>[4x]MSDSLLVRTSRDGDQFHYLWAARRALRLLEPQSTLVALTIEGASTTEMGSQPVVEDGEELIDIAEYYGSNELATATTVRYMQLKHSTMHSDTPFPPSGLQKTIEGFATRYKALIQKIPVETLRTKLEFWFVTNRPVSSSFSEAINDAANQHVTRHPHDLAKLEKFTGLQGAELSIFCQLLHIEGQQDDLWSQRNILLRESAGYLPDLDTEAPLKLKELVNRKALTESAANPSITRMDVLRALGVDETDLFPAPCRIERIENSVSRTQEATLVQRVVEAFGAPVIIHADAGVGKSIFSTHIEEHLPTGSVSILYDCFGLGQYRNASSYRHHHRTALVQMANEMASRGLCHPLIPNAGTG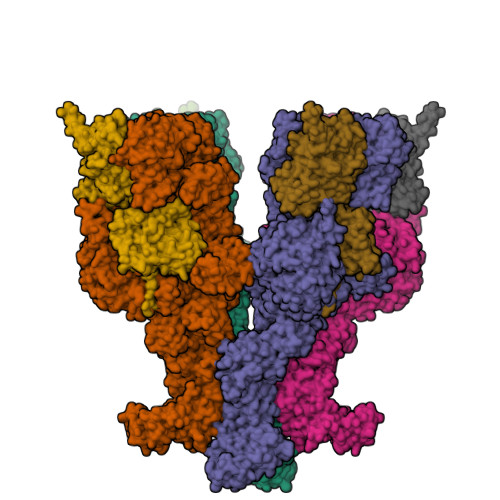ISQYMRAFLHRLSQSISILRASEPLAVLCIIIDAADNAQMAAEEIGETRSFIKDLIREKLPDGVCLVALCRPYRRELLDPPPEALTLSLQTFNRDETAAHLHQKFPDASESDVDEFHRLSSCNPRVQALSLSQNLPLNDTLRLLGPNPKTVEDTIGEVLEKSIARLRDTAGISERAQIDTICSALAILRPLIPLSVLSAISGVAGSAIKSFALDLGRPLIVSGETIQFFDEPAETWFQRRFRPSAADLHQFITKLRPLTKDSSYAASVLPALMLEGNQLSELIELAISSQALPETSAVERRDIELQRLQFALKAALRTGRYQDAAKLALKAGGECAGDNRQRVLLRDNIDLAAKFVGSNGVQELVSRNAFPDTGWPGSRNAYYAAILSEYPELSGEARSRLRLTMEWLTNWSQLPDDERSRQNVTDQDRAVMLIACLNIHGAEAAARELRRWRPRKLSFDAGKIVAMQLLAHARYDELDQLAIAAGNDISLVMGIVLEARKLHRPVAEQAIRRTWRLLKSQRVSIKDRNHANNQTIAAITGMVEMALIQSVCTESESIQLLDRYLPKVPPYALTSEYSKERVAYVRAYALQANLMGSQLALSDLASTEVKKELMAEKRHGESDDLRQLKQYSGVLIPWYNLWAKVILGKTRKADLESELSDTQKESTAIKGHSYSEHSLSSNEIANVWFDILIEAGNVSKDDVENIIKWSQHKGNRVFTPTLHRFSSVCAEISGLGELSYHFAELALSLWRDEHSDAQIKADGYIDLSRSLISLDEPEAKEYFNQAIEVTNKLGDENLSRWEAILDLAEYVAGKTQVPPEISYKLARCAELTREYVDRDKHFAWSDTVEILAELCPSSALAIISRWRDRTFGNHRSILAWTIEHLVKKNKINALDALPLITFENDWHKCDLLDSVLSSCTDDKDKIMAFEVVYHYTKFNVQNIQNLKKLDAISTSLGIEHTELKERISGLQHTETVSKKSSLSSNDNEQGHDQEWESIFKDCDLSSIDGISAAYEKFRNVPEFYSKETFIKKAISRVKTGKECSFITAIGAIFHWGLYDFKYILESIPDEWTSRLSIKTTLAGLIKEYCQRFCMRIRKSRVYEIFPFSLASRLSGISEKEIFGITLEAIAESPEPANSDRLFSLPGLLVSKLESNEALDVLSYALDLFDEVLKDEDGDGPWNEKLSPPTHVEDSLAGYIWARLGSPEAEMRWQAAHAVLALCRMSRTCVIQGIFQHAINATTLPFCDRNLPFYTLHAQLWLMIAAARVALDDGKSLIPNIGYFYHYATTDQPHVLIRHFAARTLLALHDSDLISIPAQEENKLRNINQSTTLPVLDKVEDHRGEDSYTFGIDFGPYWLKPLGRCFGVSQKQLEPEMLRIIRDVLGFKGSRNWDEDERNKRRYYQDRDNHHSHGSYPRVDDYHFYLSYHAMFMTAGQLLATKPLVGSDYDDVEDVFQDWLRRHDISRNDHRWLADRRDIPPKERSSWLNSSSDNRDEWLASISENVFNETLCPSPGLLTLWGRWSDVCSDRKESIIVHSALVSPERSLSLLRALQTTKNVYDYKIPDAGDNLEIDHAHYQLKGWIKDIAEYCGIDEFDPWAGNVRFPIPEPASFIIDAMKLTTDKDHRVWYSPSDVEPAMISSIWGHLSGKNDEEKSHGYRLCASIHFIKSALETFNMDLILEVDVDRYSRNSRYERNNENELDNIPSSTRLFLFRHDGTIHTLYGNYRNGEKTS;>[4x]MSQSQEAKNALIIAQLKGDFVAFLFVLWKALNLPKPTKCQIDMARTLANGDHKKFILQAFRGIGKSFITCAFVVWVLWRDPQLKVLIVSASKERADANSIFIKNIIDLLPFLSELKPRPGQRDSVISFDVGLAKPDHSPSVKSVGITGQLTGSRADIIIADDVEVPGNSSTSSAREKLWTLVTEFAALLKPLPTSRVIYLGTPQTEMTLYKELEDNKGYSTVIWPAQYPRNDAEALYYGDRLAPMLKAEYDEGFELLRGQPTDPVRFDMDDLRERELEYGKAGYTLQFMLNPNLSDAEKYPLRLRDAIVCAVDPERAPLSYQWLPNRQNRNEELPNVGLKGDDIHAFHTCSSRTAEYQSKILVIDPSGRGKDETGYAVLYSLNGYIYLMEVGGFRGGYDDATLEKLAKKAKQWKVQTVVHESNFGDGMFGKIFSPILLKHHKCALEEIRAKGMKEMRICDTIEPLMGAHKLVIRDEVIREDYQTARDLDGKHDVRYSAFYQMTRMTRERGAVAHDDRIDAIALGIEYLREGMLVDSRVGEEEMTLEFLEHHMEKQTIGGDQIHSFDVGGVDIYYEDEDGGSSFIEW>SEKIIHLTDDSFDTDVLKADGAILVDFWAEWCGPCKMIAPILDEIADEYQGKLTVAKLNIDQNPGTAPKYGIRGIPTLLLFKNGEVAATKVGAL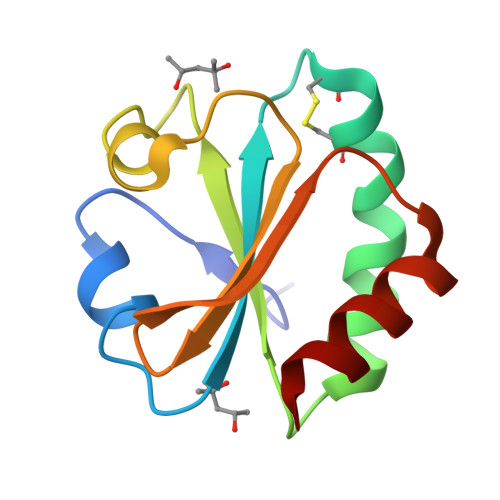SKGQLKEFLDANLA[2x]>[4x]MASHASCIFCK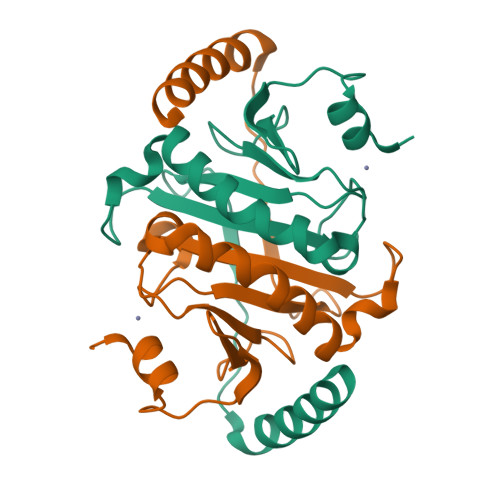IIKGEIPSFKLIETAKTYSFLDIQPIAEAHVLIIPKHHGAKLHNIPDDYLSDILPVVKKLTKVLKLDENNTPEGEGYNVLQNNGRIAHQVVDHVHFHLIPKKDEATGLGVGWPAEATDFDKLGKLHEKLKEELAKVDEEKLLEHHHHHH N-(4-{[3-(1-methyl-1H-pyrazol-4-yl)-1H-indol-5-yl]oxy}phenyl)glycinamide | C20 H19 N5 O2 | 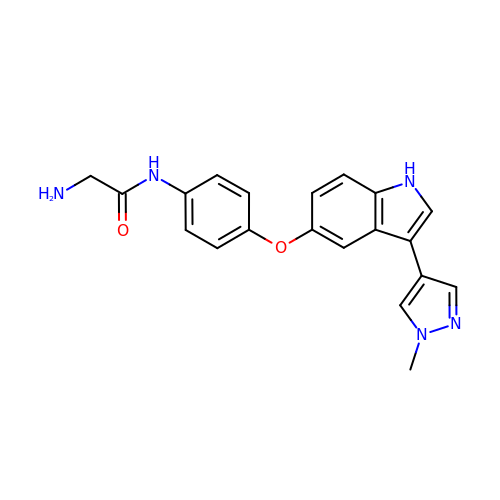HGVGFSWIDYRBBA-UHFFFAOYSA-N> YIPEWEGRAPDSVD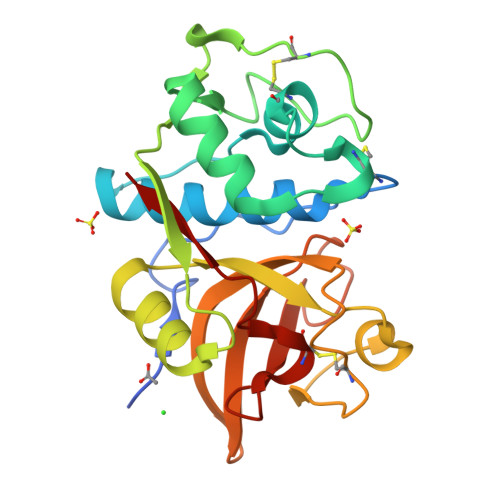YRKKGYVTPVKNQGQCGSSWAFSSVGALEGQLKKKTGKLLNLSPQNLVDCVSENDGCGGGYMTNAFQYVQKNRGIDSEDAYPYVGQEESCMYNPTGKAAKCRGYREIPEGNEKALKRAVARVGPVSVAIDASLTSFQFYSKGVYYDESCNSDNLNHAVLAVGYGIQKGNKHWIIKNSWGENWGNKGYILMARNKNNACGIANLASFPKM[(2R,3R,4S,5S)-5-(2-azanyl-6-oxidanyl-purin-9-yl)-3,4-bis(oxidanyl)oxolan-2-yl]methyl bis(oxidanyl)phosphinothioyl hydrogen phosphate | C10 H15 N5 O10 P2 S | 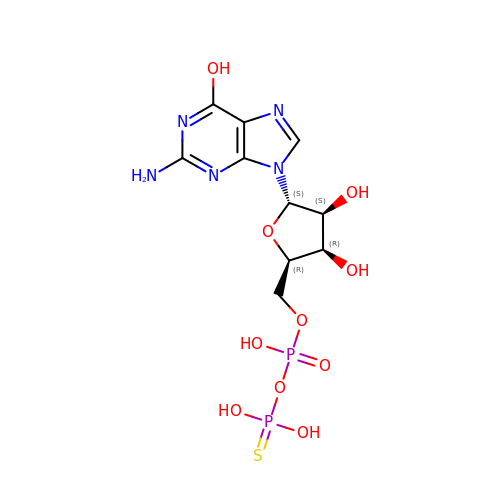QJXJXBXFIOTYHB-KHLHZJAASA-N>MAIGLPSINISFKELATTVKERSARGIIAMVLKDAKALGLNEIHEKEDIPVDLSAENKEYINLALMGNVNTPNKLLVYVIEGEADIQTALDFLETKEFNYLCMPKAVEADKTAIKNWIIKLRDIDKVKVKAVLGKVVGNHEGIINFTTEDVLVGEKKYSVDEFTSRVAGLIAGTPLSQSVTYTKLSDVVDIPKMTKVDAESRVNKGELILIKEAGAIRIARGVNSLTELTAEKGEMFQKIKIVDTLDIIHSDIRKVIIDDYIGKVTNSYDNKCLLIVAIKSYLEELEKSALIESDSTVEIDFEAQKSYLKSKGVDLSYMTLQEIKEANTGSKVFLKAKIKVLDAMEDIDLSIEI[18x];>MLKYKEILETIIEILKKNFTESIFIDDESVQGSEGSCFFVSILSVICTPVMLNTNNKDIVISIKYLPKPQSKSIRMYEISDELNKLFNRNIKVTDRKLNITKLEQSIKKEESIYVLNFTFTLNYLDSVYEEDVVYENMKEINLNLGE[6x];>MANMEARNVMSGTWGELWLDGNKVAEVKKFQAKMEFTKEDIIIAGQMGTDTKYMGYKGKGSITLYHVSSRMHKLIGEKIKRGSEPRFVAISKLNDPDSYGAERIAVKNIAFDDLTLADWEVGVKGEIEAPFTF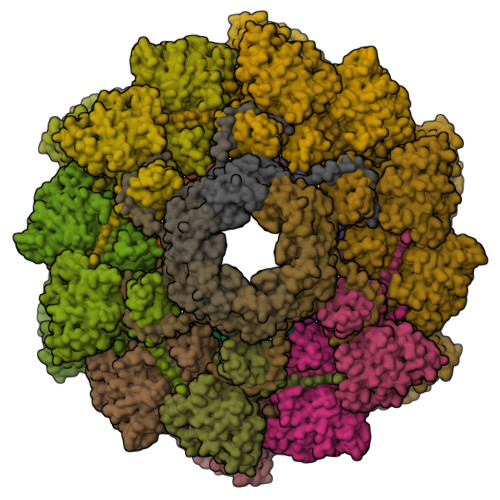TEYDFLDII[18x]>SEFELRRQACGRSQLLKSRVDILEVARQFEMRINLDIVDSMIASAIENNKVATEILPPVETLRSRQFEASKLREIRKNIDSGFYTQEEIEVIARSMLDDVAELSSDYLGNTVVQKFFEYCSDPIKEAMLERIAPYLAAIGIHKNGTWAAQKIIDVASTEKQMDLIVKHLRPYTALLYFDQFGNYVAQCCLRFKYPKNTFLFEVMARHCCEIGQSRFGARAIRACLENENATFEQQALVVASIIINSHLLATNSNGMLLLTWLLDNSFFRNRHRLLAIHLATHL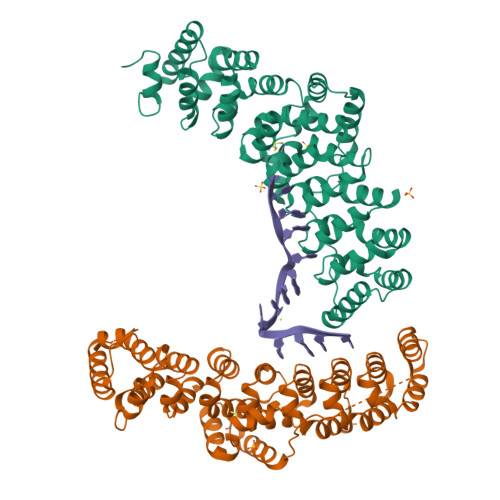HTTCTHKLASTLIFKLINNKQEPESRNLLLKNLFFSEKDNVLTYILQDQAVGPSFIHKVITYPSIGREFLAQFHLVIKRVLINIHAQPNAVYCRLMEEVGMTSKSI[2x]> MKLAMIGFGQAGGKVVDKFVEYDRERNAGIVRAAVAVNSAKADLLGLKNIPKDQRVLIGQSRVKGHGVGADNELGAEIAEEDIDEVQGAIDSIPVHEVDAFLVVSGLGGGTGSGGAPVLAKHLKRIYTEPVYGLGILPGSDEGGIYTLNAARSFQTFVREVDNLLVFDNDAWRKTGESVQGGYDEINEEIVNRFGVLFGAGEVQDGQEVAESVVDSSEIINTLAGGGVSTVG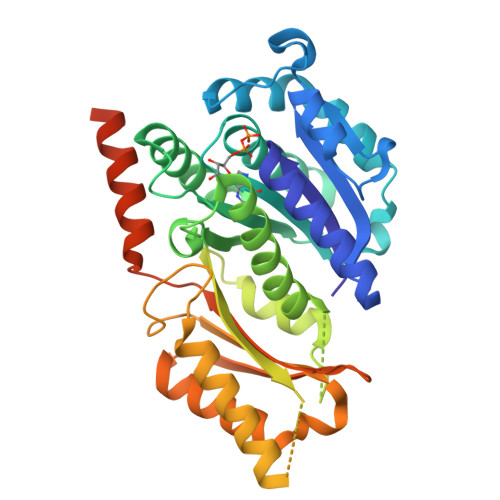YASEGVEPRKNNGGGLLSRLTGGDEPDDNLDTAHTTNRITSLVRKAALGRLTLPCEIEGAERALLVLAGPPEHLNRKGIERGRKWIEEQTGSMEVRGGDYPIPGAEKVAGVILLSGVTNVPRIKELQQVAIEAQDNIEEIRQESDSNLETLINDDEDELESLF> QASVE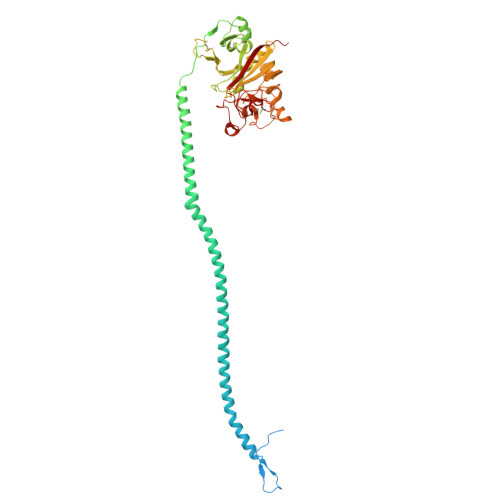YDNEEDSPQIDARAHRPLDKRQEAAPTLRPVAPPISGTGYQPRPPKQDKQAMKKGPIIYPDAGGCKHPLDELGVLCPTGCELQTTLLKQEKTVKPVLRDLKDRVAKFSDTSTTMYQYVNMIDNKLVKTQKQRKDNDIILSEYNTEMELHYNYIKDNLDNNIPSSLRVLRAVIDSLHKKIQKLENAIATQTDYCRSPCVASCNIPVVSGRECEDIYRKGGETSEMYIIQPDPFTTPYRVYCDMETDNGGWTLIQNRQDGSVNFGRAWDEYKRGFGNIAKSGGKKYCDTPGEYWLGNDKISQLTKIGPTKVLIEMEDWNGDKVSALYGGFTIHNEGNKYQLSVSNYKGNAGNALMEGASQLYGENRTMTIHNGMYFSTYDRDNDGWLTTDPRKQCSKEDGGGWWYNRCHAANPNGRYYWGGTYSWDMAKHGTDDGIVWMNWKGSWYSMKKMSMKIKPYFPD>[2x]MIPQTLEQLLSQAQSIAGLTFGELADELHIPVPIDLKRDKGWVGMLLERALGATAGSKAEQDFSHLGVELKTLPINAEGYPLETTFVSLA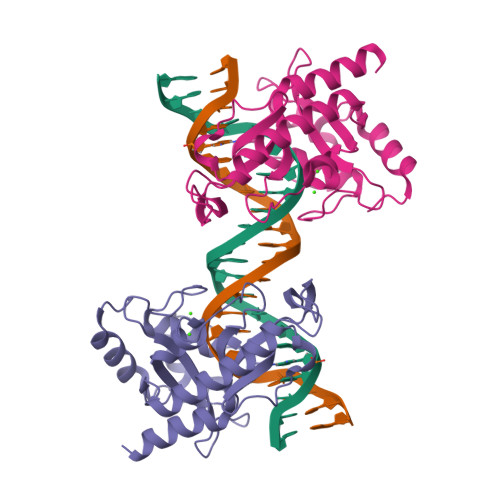PLVQNSGVKWENSHVRHKLSCVLWMPIEGSRHIPLRERHIGAPIFWKPTAEQERQLKQDWEELMDLIVLGKLDQITARIGEVMQLRPKGANSRAVTKGIGKNGEIIDTLPLGFYLRKEFTAQILNAFLETKSL> MAHHHHHHMGTLEAQTQGPSMTKPDLASLEKTIEKAFDERDGINTATRGEVREAVEQSLILLDRGEVRVAEKQADGNWHVNQWLKKAVLLSFRLNPMEVIKGGPGQSSWWDKVPSKFDGWTANEFEKAGFRAVPNCIVRHSAYIAPNAILMPSFVNLGAYV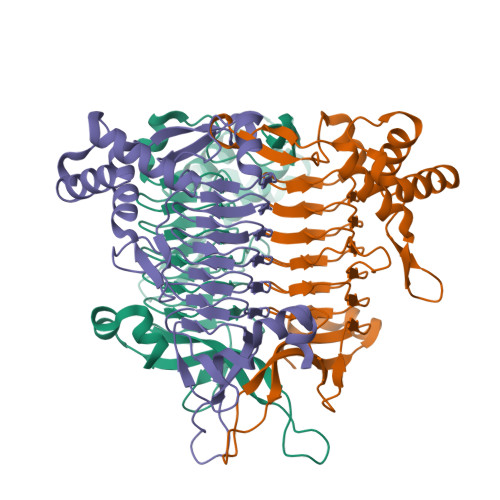DKGAMIDTWATVGSCAQIGKNVHLSGGVGIGGVLEPMQAGPTIIEDNCFIGARSEVVEGCIVREGSVLGMGVFIGKSTKIVDRATGEVFYGEVPPYSVVVAGTMPGKNVPGENWGPSLYCAVIVKRADEKTRSKTSINELLRD>[2x]MQERRALRLGVNGLPNSLEPVNAISNVGPRIVNQIFDTLIARDFFAKGAPGNAIDLVPALAESWERIDEKSVRFKLRQKVMFHDGVELTADDVAYTFSSERLWGPEAIKKIPLGKSYSLDFDEPVVEDKYTVTLRTKTPSYLIETFVASWMSRIVPKEYYKKLGAVDFGNKPVGTGPYKFVEFVAGDRVVLEANDAYWGPKPTASKITYQIVAEPATRVAGLISGEYDIITTLTPDDIQLINSYPDLETRGTLIENFHMFTFNMNQEVFKDKKLRRALALAVNRPIMVEALWKKQASIPAGFNFPNYGETFDPKRKAMEYNVEEAKRLVKESGYDGTPITYHTMGNYYANAMPALMMMIEMWKQIGVNVVMKTYAPGSFPPDNQTWMRNWSNGQWMTDAYATIVPEFGPNGQVQKRWGWKAPAEFNELCQKVTVLPNGKERFDAYNRMRDIFEEEAPAVILYQPYDVYAARKDVHWKPVSFEMMEFRNNLSFGHHHHHH

To our knowledge, the best known system that exemplifies this paradigm is the antibiotic agrocin 84, which penetrates into the cytoplasm of the bacterial pathogen Agrobacterium tumefaciens strain C58 by hijacking the PBP called AccA and its cognate transporter. AccA also plays a key-role in the importation of the characteristic plant tumour-derived compounds such as the opines agrocinopines A and B discovered in 1981 in crown gall tumour tissue. The mature AccA structure is a monomer of 493 residues composed of two lobes, each formed by a central β-sheet flanked by α-helices. We identified the pyranose-2-phosphate-like moiety shared by these two ligands as the key recognition template for AccA.

A better resolution structure of this complex at 1.9 Å resolution in a different space group using the native protein was determined. The two agrocinopine-complexed structures are very similar, displaying an average root mean square deviation (rmsd) of 0.35 Å over 489 Cα atoms. Overall, the ligand bound structures are very similar (average rmsd value of 0.33 Å over 490 Cα atoms) adopting a closed conformation. The major difference concerns the region comprising the residues 403–408, which can move up to 1.7 Å to accommodate the ligand in the binding site. While Agrocinopine A is fully defined in the electron density maps, the leucine-like moiety of agrocin 84 is mobile. It makes extensive protein hydrogen bonds: 8 for L-arabinose and 10 for D-glucose. In contrast, the sucrose moiety of agrocinopine A and the TM84 part of agrocin 84 make only 3 and 2 polar interactions with AccA, respectively. A particularity of AccA which is not shared by these related PBPs is the presence of the flexible loop 402–414 located between the β-strands β15 and β16 which can accommodate agrocinopine A. This loop corresponds to a conserved rigid helix in all similar PBPs and models superposition shows that an equivalent helix in our structure would clash with the last glucose of agrocinopine A.>[2x]MTDMWDVRITDTSLRDGSHHKRHQFTKDEVGAIVAALDAAGVPVIEVTHGDGLGGSSFNYGFSKTPEQELIKLAAATAKEARIAFLMLPGVGTKDDIKEARDNGGSICRIATHCTEADVSIQHFGLARELGLETVGFLMMAHTIAPEKLAA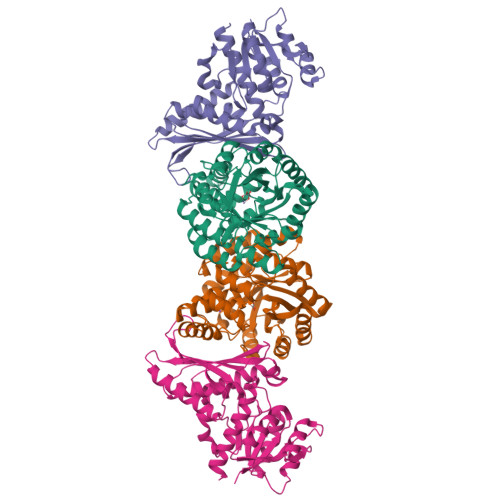QARIMADAGCQCVYVVDSAGALVLDGVADRVSALVAELGEDAQVGFHGHENLGLGVANSVAAVRAGAKQIDGSCRRFGAGAGNAPVEALIGVFDKIGVKTGIDFFDIADAAEDVVRPAMPAECLLDRNALIMGYSGVYSSFLKHAVRQAERYGVPASALLHRAGQRKLIGGQEDQLIDIALEIKRELDSGAAVTH;>GSHMPSKAKVAIVGSGNISTDLLYKLLRSEWLEPRWMVGIDPESDGLARAAKLGLETTHEGVDWLLAQPDKPDLVFEATSAYVHRDAAPKYAEAGIRAIDLTPAAVGPAVIPPANLREHLDAPNVNMITCGGQATIPIVYAVSRIVEVPYAEIVASVASVSAGPGTRANIDEFTKTTARGVQTIGGAARGKAIIILNPADPPMIMRDTIFCAIPTDADREAIAASIHDVVKEVQTYVPGYRLLNEPQFDEPSINSGGQALVTTFVEVEGAGDYLPPYAGNLDIMTAAATKVGEEIAKETLVVGGAR[2x]> MAIYADNSYSIGNTPLVRLKHFGHNGNVVVKIEGRNPSYSVKCRIGANMVWQAEKDGTLTKGKEIVDATSGNTGIALAYVAAARGYKITLTMPETMSLERKRLLCGLGVNLVLTEGAKGMKGAIAKAEEIVASDPSRYVMLKQFENPANPQIHRETTGPEIWKDTDGKV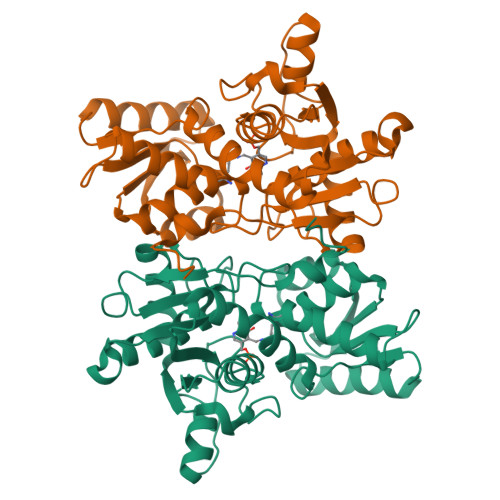DVVVAGVGTGGSITGISRAIKLDFGKQITSVAVEPVESPVISQTLAGEEVKPGPHKIQGIGAGFIPKNLDLSIIDRVETVDSDTALATARRLMAEEGILAGISSGAAVAAADRLAKLPEFADKLIVVILPSAGERYLSTALFEGIEG> SKRVEVLLTQLPAYNRLKTPYEAELIETAKKMTAPGKGLLAADESTGSCSKRFAGIGLSNTAEHRRQYRALMLECEGFEQYISGVILHDETVYQKAKTGETFPQYLRRRGVVPGIKTDCGLEPLVEGAKGEQMTAGLDGYIKRAKKYYAMGCRFCKWRNVYKIQNGTVSEAVVRFNAETLARYAILSQLCGLVPIVEPEVMIDGT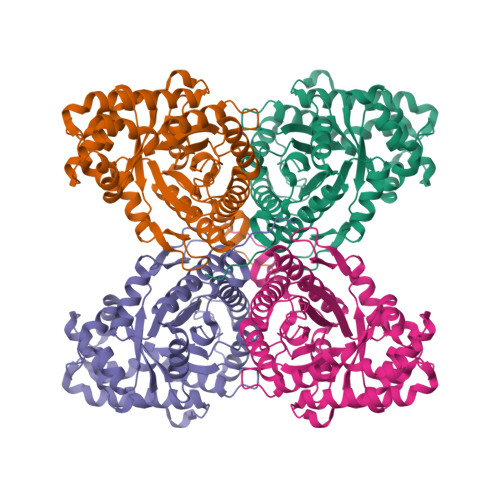HDIETCQRVSQHVWSEVVSALHRHGVVWEGCLLKPNMVVPGAESGLKGHAEQVAEYTVKTLARVIPPALPGVTFLSGGLSEVMASEYLNAMNNCPLPRPWKLTFSYARALQSSAIKRWGGKESGVEAGRRAFMHRAKMNSLAQLGKYNRADDDKDSQSLYVAGNT> GSNNHHLYPDELNVSNNPHYRPKPVSYDSTLPPDHIKVYSRTLFIGGVPLNMKEWDLANVLKPFAEVQSVILNNSRKHAFVKVYSRHE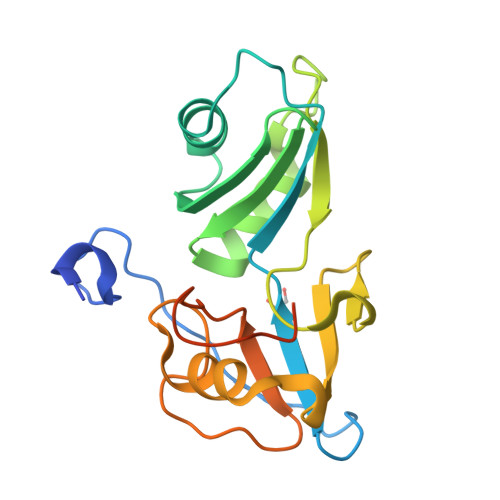AENVLQNFNKDGALPLRTRWGVGFGPRDCCDYQHGYSIIPMHRLTDADKKWSVSAQWGGTSGQPLVTGIVFEEPDIIVGEGVSSKAISQKMPTDSGRNGPRSG MCR-1 confers resistance by modifying the colistin target, catalyzing transfer of phosphoethanolamine (PEA) onto the glucosamine saccharide of lipid A in the bacterial outer membrane. Bacterial lipooligosaccharide PEA-transferases such as MCR-1 are organised into two domains: an N-terminal inner membrane-bound domain predicted to contain 5 transmembrane α-helices and a soluble, periplasmic domain containing the putative catalytic centre. Here we present two crystal structures of the soluble, catalytic domain of MCR-1, revealing this to be a zinc metalloprotein containing three intramolecular disulphide bonds. The two structures are essentially identical (RMSD 0.37 Å over 311 Cα atoms) and reveal an overall α-β-α fold, containing three intramolecular disulphide bonds, typical of alkaline phosphatase or sulphatase enzymes, with the N-terminus indicating the likely position of the five transmembrane helices.

To facilitate such studies, we engineered MCR-1 to lack the five transmembrane helices, generating a construct containing residues 219–541 (MCR1ΔTM) which was purified and crystallised. Phases calculated from datasets collected at or near the zinc X-ray absorption edge ultimately yielded structures for two different crystal forms in the space groups P41212 (1.75 Å resolution) and P21 (1.55 Å resolution). However, the two crystal forms differ in zinc content, with the P21 structure containing one zinc ion (Zn1), coordinated by Asp465, His466, Glu246 and Thr285 in a tetrahedral geometry, while the P41212 structure contains density for an additional, also tetrahedral, zinc site (Zn2) coordinated by His395, His478, a water molecule (Wat1) and Glu300 from a symmetry related molecule. Furthermore, the active site of the P21 structure contains electron density corresponding to the presence of a phosphate group attached to Thr285, the conserved residue believed to act as the acceptor for the PEA group during the transfer reaction. This apparent autophosphorylation was confirmed by mass spectrometry of MCR1ΔTM crystallisation samples, which showed a mixed population of proteins with a mass difference (78 Da) consistent with the presence of phosphorylated and non-phosphorylated forms. In particular, in addition to their possible roles as Zn2 ligands (P41212 structure), in the P21 structure both His395 and His478 are well positioned to interact with phosphorylated Thr285, whilst the proximity of Lys333 to Thr285 suggests a possible role for this residue in substrate (PEA) binding. Moreover, both comparisons with previous structures, and our observation of phosphorylation in one of our two structures, clearly identify Thr285 as the likely nucleophile and PEA acceptor in the catalytic mechanism. For the mono-zinc mechanism, a model containing Glu246, Thr285, Asp465 and His466, with both Glu246 and Asp465 deprotonated, provided the best agreement with the experimental crystal structure.

>GPTIYHAKDAVQATKPDMRKPRLVVFVVGETARADHVSFNGYERDTFPQLAKIDGVTNFSNVTSCGTSTAYSVPCMFSYLGADEYDVDTAKYQENVLDTLDRLGVSILWRDNNSDSKGVMDKLPKAQFADYKSATNNAICNTNPYNECRDVGMLVGLDDFVAANNGKDMLIMLHQMGNHGPAYFKRYDEKFAKFTPVCEGNELAKCEHQSLINAYDNALLATDDFIAQSIQWLQTHSNAYDVSMLYVSDHGESLGENGVYLHGMPNAFAPKEQRSVPAFFWTDKQTGITPMATDTVLTHDAITPTLLKLFDVTADKVKDRTAFIR[2x]> EFMVSLPRMVYPQPKVLTPCRKDVLVVTPWLAPIVWEGTFNIDILNEQFRLQNTTIGLTVFAIKKYVAFLKLFLETAEKHFMVGHRVHYYVFTDQPAAVPRVTLGTGRQLSVLEVGAYKRWQDVSMRRMEMIS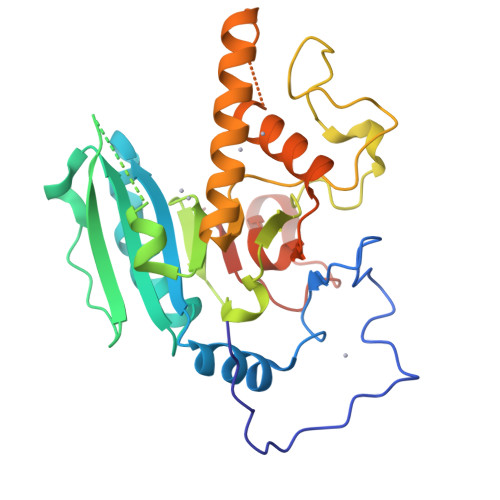DFCERRFLSEVDYLVCVDVDMEFRDHVGVEILTPLFGTLHPSFYGSSREAFTYERRPQSQAYIPKDEGDFYYMGAFFGGSVQEVQRLTRACHQAMMVDQANGIEAVWHDCSHLNKYLLRHKPTKVLSPEYLWDQQLLGWPAVLRKLRFTAVPKNHQAVRNPE> DVSFRLSGATSSSYGVFISNLRKALPNERKLYDIPLLRSSLPGSQRYALIHLTNYADETISVAIDVTNVYIMGYRAGDTSYFFNEASATEAAKYVFKDAMRKVTLPYSGNYERLQTAAGKIRENIPLGLPALDSAITTLFYY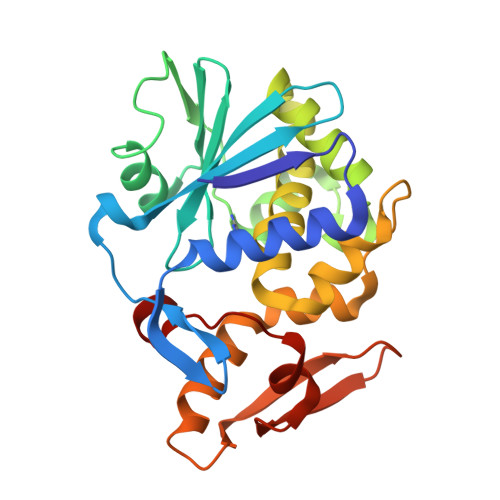NANSAASALMVLIQSTSEAARYKFIEQQIGKRVDKTFLPSLAIISLENSWSALSKQIQIASTNNGQFESPVVLINAQNQRVTITNVDAGVVTSNIALLLNRNNMA>MFTGSIVAIVTPMDEKGNVCRASLKKLI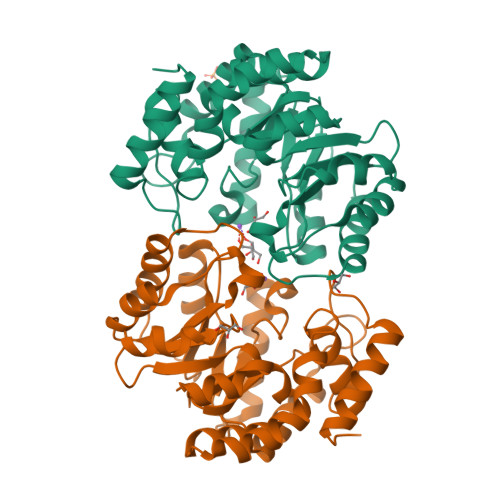DYHVASGTSAIVSVGTTGESATLNHDEHADVVMMTLDLADGRIPVIAGTGANATAEAISLTQRFNDSGIVGCLTVTPYYNRPSQEGLYQHFKAIAEHTDLPQILYNVPSRTGCDLLPETVGRLAKVKNIIGIREATGNLTRVNQIKELVSDDFVLLSGDDASALDFMQLGGHGVISVTANVAARDMAQMCKLAAEGHFAEARVINQRLMPLHNKLFVEPNPIPVKWACKELGLVATDTLRLPMTPITDSGRETVRAALKHAGLL[2x]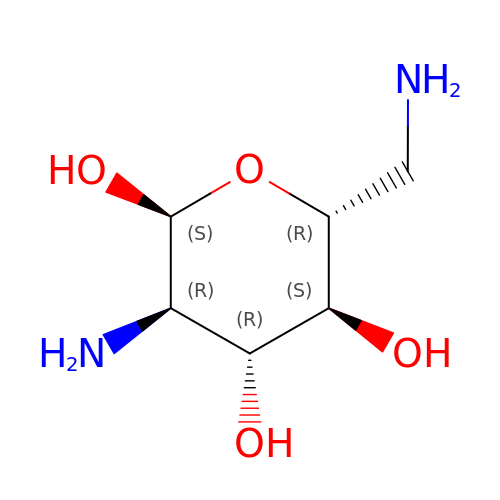2,6-diamino-2,6-dideoxy-alpha-D-glucopyranose | C6 H14 N2 O4 | SQTHUUHOUPJYLK-UKFBFLRUSA-N>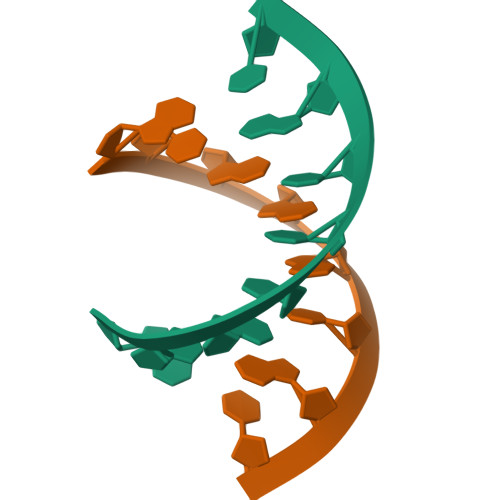 GUGUUUAC;> GUAGGCAC>[2x]HHHHHHGSMGFLILSRREGEGITLSLKADY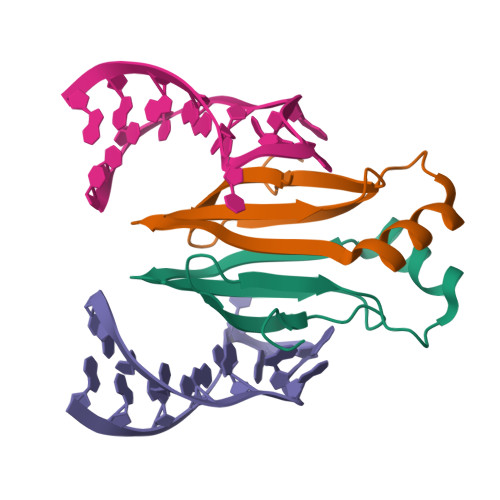PAEELIRQLREGGIRILVTDIIGNQARVGIEAPRGVLIVRDELKTAPKG>[2x]TRINLT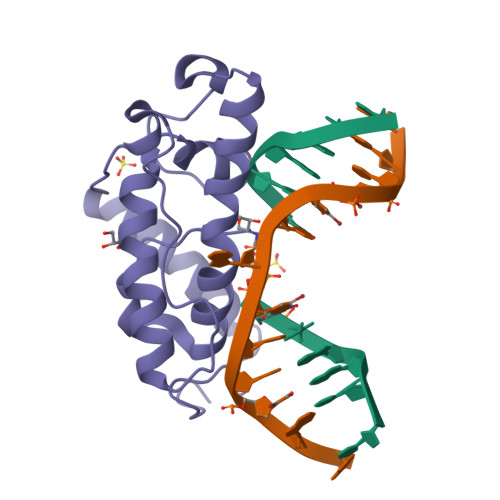LVSELADQHLMAEYRELPRVFGAVRKHVANGKRVRDFKISPTFILGAGHVTFFYDKLEFLRKRQIELIAECLKRGFNIKDTTVQDISDIPQEFRGDYIPHEASIAISQARLDEKIAQRPTWYKYYGKAIYA3-METHYLTHIAZOLIUM 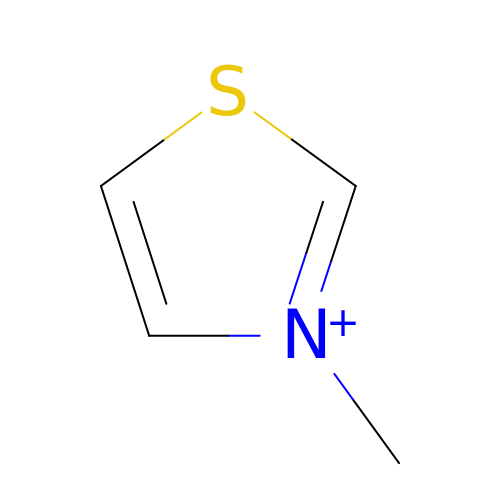ION | C4 H6 N S | PIDRHKDECUFWTG-UHFFFAOYSA-N>MSRLDKSKVINSALELLNEVGIEGLTTRKLAQKLGVEQPTLYWHVKNKRALLDALAIEMLDRHHTHFSPLEGESWQDFLRNNAKSFRNALLSHRDGAKVHLGTRPTEKQYETLENQLAFLTQQGFSLENALYALSAVGHFTLGSVLEDQEHQVAKEERET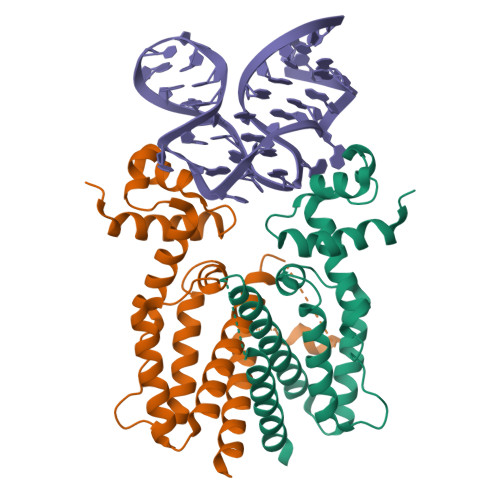PTTDSMPPLLRQAIELFDHQGAEPAFLHGLESLIRGFEVQLTALLQIV[2x]>CGCXAATTXGC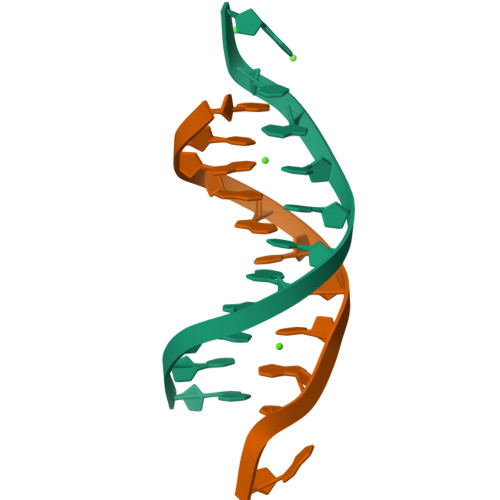G[2x]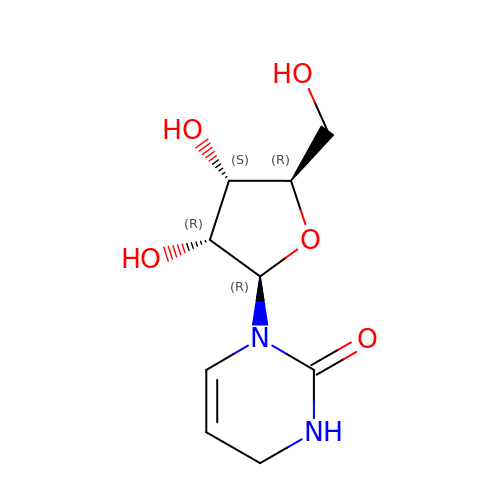3,4-DIHYDRO-1H-PYRIMIDIN-2-ONE NUCLEOSIDE | C9 H14 N2 O5 | NVRAAJMSMZQKRW-WCTZXXKLSA-N> MS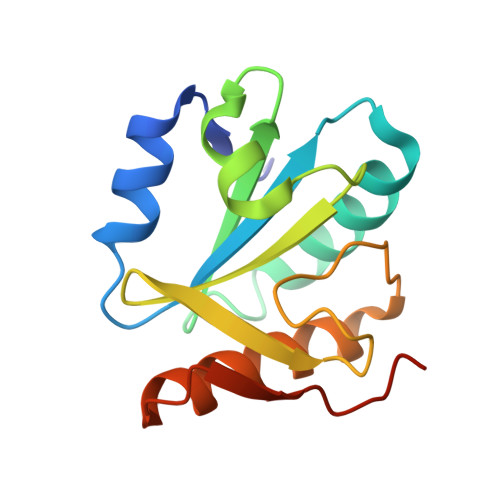YMLPHLHNGWQVDQAILSEEDRVVVIRFGHDWDPTCMKMDEVLYSIAEKVKNFAVIYLVDITEVPDFNKMYELYDPCTVMFFFRNKHIMIDLGTGNNNKINWAMEDKQEMVDIIETVYRGARKGRGLVVSPKDYSTKYRY> WSHPQFEKGAETAVPNSEDVMKRAQGLFKPIPAKPPVMKDNPASPSRVELGRMLFFDPRLSASHLISCNTCHNVGLGGTDI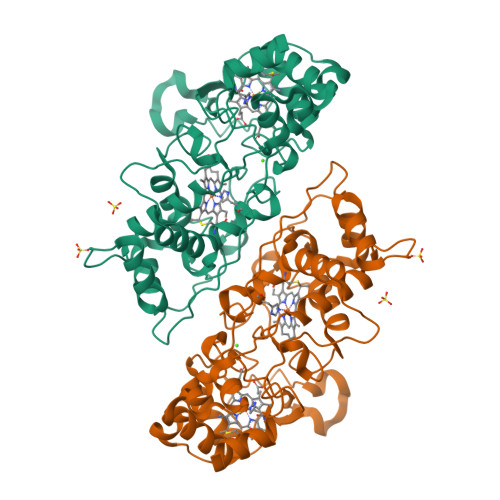LETSIGHGWQKGPRNSPTVLNAVYNIAQFWDGRAEDLAAQAKGPVQASVEMNNKPENLVATLKSIPGYPPLFRKAFPGQGDPVTFDNVAKAIEVFEATLVTPDAPFDKYLKGNRKAISSTAEQGLALFLDKGCAACHSGVNMGGTGYFPFGVREDPGPVVRPVDDTGRYKVTSTAADKYVFRSPSLRNVAITMPYFHSGKVWKLKDAVKIMGSAQLGISITDADADKIVTFLNTLTGAQPKVMHPVLPPNSDDTPRPVSN>MINDRSDHGTGTARVGQVKEVTSLTNPIVKDIRALTQKKHRDETRSFMAEGLKLVIDALDLGWKIKTLVYAKAAKGKPQVEQVAAKTVARGGLVLEVNEKVISTITRRDNPQMVVGIFEQRYSPLRDIHPQEGETYVALDRVRDPGNLGTIIRTADAAGASGIILVGETTDPFSLETVRATMGSVFAIPIARANTEDFIRWQRAAGVQVVATHLAGSVDYRTIDYKSKPVVLLMGNEQAGLPVELAREAGALARIPQAGRADSLNLAIATGIML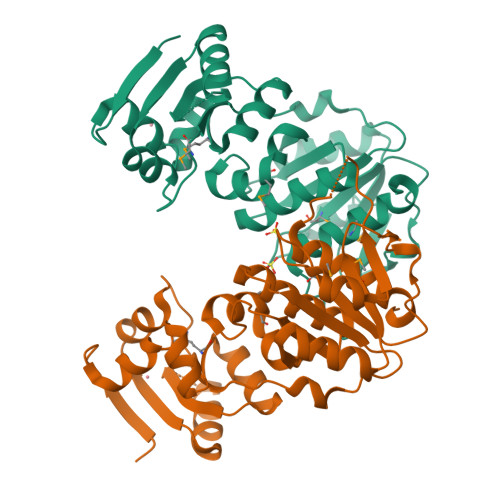FEARRHLLSLDGGR[2x]>[2x]MADQQTTMPRWVPLLLGLLGSTTCGMLLYAWSVFIKPLNAEFGWSRAEIAMAFAICCLIFGLMTFPAGRLSDKMGPRKVVMTGGVLLAIGFILSGFIQSKYQLYITYGVIAGFGGGMIYLPPIATAPKWWPDRRALATGFAVVGLGLGSFLMGPLATYIIEKPGM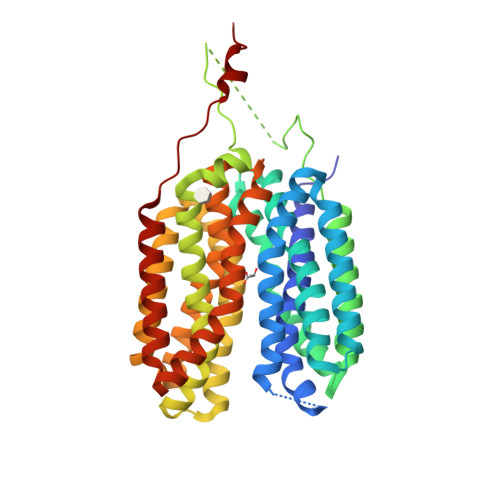GWRYVFWYCGVAMGIMALIAGAFLEPPPAGWKPAGYTPPAPPAGAAAPKVTRDWTYEEAKGDTKFWLLYLAYFCGSFAGLMVIGHLAGFGRDAGLTAMAAAGAVSSLAFSNAATRILSGWFVDKIGIRVYFAALFALQTAAMIAIFQLGGSVVGLSIVAIVIGWNYGAMFTLFPATCLQFYGPTAQGSNYGLLFTACGLAGFAGPWVGGWLKDTTGTYYLPFLCAAALCALGTAIVFMTKPPEKKHALELEVLFQ>MLGGLLHRGHKIKGTVVLMRKNVLDVNSVTSVGGIIGQGLDLVGSTLDTLTAFLGRSVSLQLISATKADANGKGKLGKATFLEGIITSLPTLGAGQSAFKINFEWDDGSGIPGAFYIKNFMQTEFFLVSLTLEDIPNHGSIHFVCNSWIYNAKLFKSDRIFFANQTYLPSETPAPLVKYREEELHNLRGDGTGERKEWERIYDYDVYNDLGDPDKGENHARPVLGGNDTFPYPRRGRTGRKPTRKDPNSESRSNDVYLPRDEAFGHLKSSDFLTYGLKSVSQNVLPLLQSAFDLNFTPREFDSFDEVHGLYSGGIKLPTDIISKISPLPVLKEIFRTDGEQALKFPPPKVIQVSKSAWMTDEEFAREMLAGVNPNLIRCLKDFPPRSKLDSQVYGDHTSQITKEHLEPNLEGLTVDEAIQNKRLFLLDHHDPIMPYLRRINATSTKAYATRTILFLKNDGTLRPLAIELSLPHPQGDQSGAFSQVFLPADEGVESSIWLLAKAYVVVNDSCYHQLVSHWLNTHAVVEPFIIATNRHLSVVHPIYKLLHPHYRDTMNINGLARLSLVNDGGVIEQTFLWGRYSVEMSAVVYKDWVFTDQALPADLIKRGMAIEDPSCPHGIRLVIEDYPYTVDGLEIWDAIKTWVHEYVFLYYKSDDTLREDPELQACWKELVEVGHGDKKNEPWWPKMQTREELVEACAIIIWTASALHAAVNFGQYPYGGLILNRPTLSRRFMPEKGSAEYEELRKNPQKAYLKTITPKFQTLIDLSVIEILSRHASDEVYLGERDNPNWTSDTRALEAFKRFGNKLAQIENKLSERNNDEKLRNRCGPV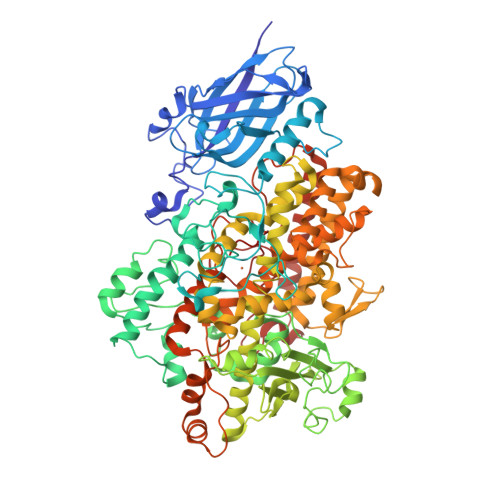QMPYTLLLPSSKEGLTFRGIPNSISI[2x]> DYKDDDDAAAQTSAPPAVSPQITVLAPGKGPWQVAFIGITTGLLSLATVTGNLLVLISFKVNTELKTVNNYFLLSLACADLIIGTFSMNLYTTYLLMGHWALGTLACDLWLALDYVASNASVMNLLLISFDRYFSVTRPLSYRAKRTPRRAALMIGLAWLVSFVLWAPAILFWQYLVGERTVLAGQCYIQFLSQPIITFGTAMAAFYLPVTVMCTLYWRIYRFRRRGAEALERAFSLEDDKEALLAALDALAEAFADDAELTALLALLRRLLEDPDLPADELAALRAALTRFPEFREALLALLDRYL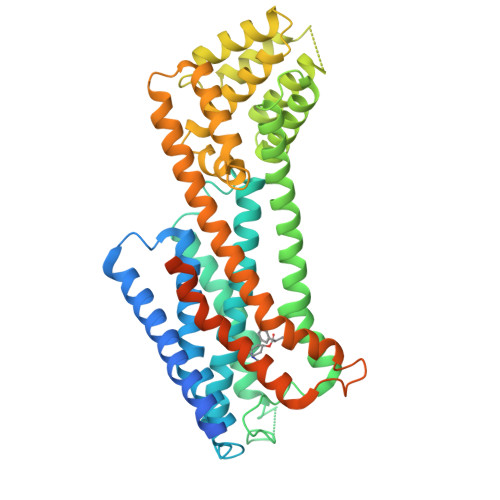ATRDLADARDLVWALVLAIASDPRYRPAVAAMIAFGDAEVLRAGLLRGAEALGLPGGEALVEEIMAEAEKEKKAARTLSAILLAFILTWTPYNIMVLVSTFCKDCVPETLWELGYWLCYVNSTINPMCYALCNKAFRDTFRLLLLCRWDKRRWRKIPKRPGSVHRTPSRQCHHHHHHHHH> VVKTAQNLAEVNGPETLIGPGAKEGTVPTDLDQETGLARLELLGKLEGIDVFDTKPLDSSRKGTMKDPIIIESYDDY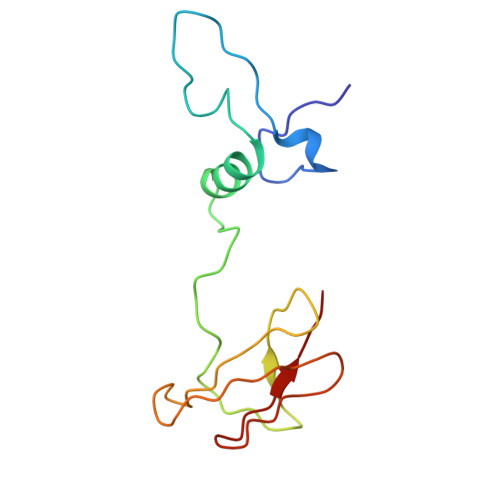RYVGCTGSPAGSHTIMWLKPTVNEVARCWECGSVYKLNPV> MGSQVSTQRSGSHENSNSASEGSTINYTTINYYKDAYAASAGRQDMSQDPKKFTDPVMDVIHEMAPPLKSPSAEACGYSDRVAQLTIGNSTITTQEAANIVIAYGEWPEYCPDTDATAVDKPT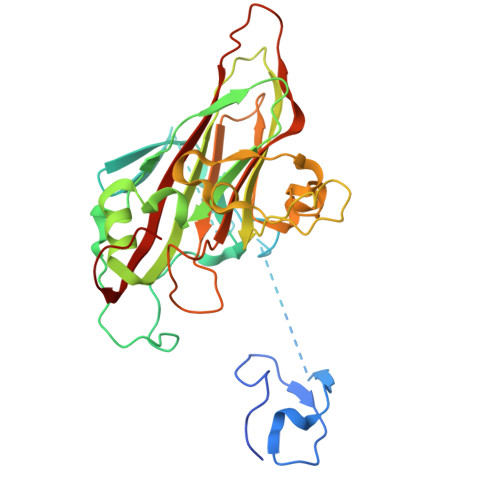RPDVSVNRFFTLDTKSWAKDSKGWYWKFPDVLTEVGVFGQNAQFHYLYRSGFCVHVQCNASKFHQGALLVAVLPEYVLGTIAGGTGNENSHPPYATTQPGQVGAVLTHPYVLDAGIPLSQLTVCPHQWINLRTNNCATIIVPYMNTVPFDSALNHCNFGLLVIPVVPLDFNTGATSEIPITVTIAPMCAEFAGLRQAVKQ> LPDSVDWREKGCVTEVKYQGSCGACWAFSAVGALEAQLKLKTGKLVSLSAQNLVDCSTEKYGNKGCNGGFMTTAFQYIIDNKGIDSDASYPYKAMDQKCQYDSKYRAATCRKYTELPYGREDVLKEAVANKGPVSVGVDARHPSFFLYRSGVYYEPSCTQNVNHGVLVVGYGDLNGKEYWLVKNSWGHNFGEKGYIRMARNKGNHCGIASFP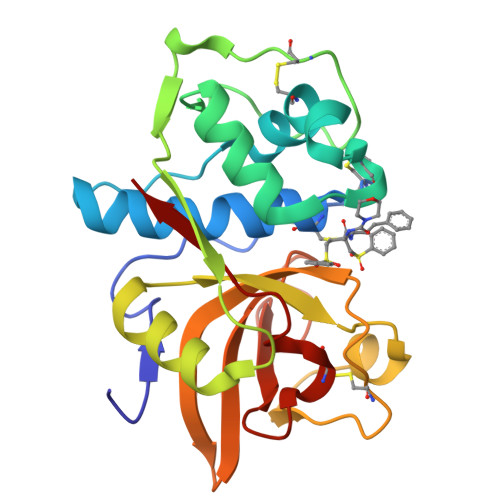SYPEI Inosine-3',5'-cyclic 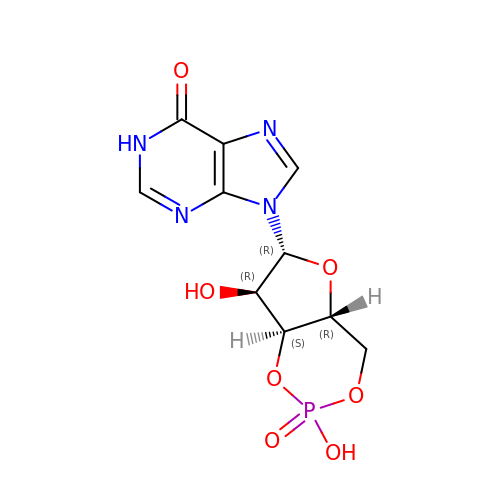monophosphate | C10 H11 N4 O7 P | DMJWGQPYNRPLGA-KQYNXXCUSA-N Collagen prolyl 4-hydroxylases (C-P4H) are α2β2 tetramers, which catalyze the prolyl 4-hydroxylation of procollagen, allowing for the formation of the stable triple-helical collagen structure in the endoplasmic reticulum. The C-P4H α-subunit provides the N-terminal dimerization domain, the middle peptide-substrate-binding (PSB) domain, and the C-terminal catalytic (CAT) domain, whereas the β-subunit is identical to the enzyme protein disulfide isomerase (PDI). C-P4Hs are Fe(II) and 2-oxoglutarate-dependent dioxygenases, which use molecular oxygen to hydroxylate proline residues that are present at the Y position of the -X-Y-Gly- repeats of the procollagen chain. Studies have shown that the β/PDI subunit is required for providing the soluble and catalytically competent conformation of the α-subunit, but it is not understood how it is assembled with the α-subunit, how it is involved in intersubunit disulfide bridges, and what its role is in the procollagen hydroxylation reaction mechanism of the mature C-P4H α2β2 tetramer.

Here, we report on the characterization of two truncated human C-P4H-II variants in which the α-subunit is lacking either the N-terminal dimerization domain (C-P4H-II-Δ140) or the dimerization domain and the PSB domain (C-P4H-II-Δ281). The asymmetric unit consists of two C-P4H-II-Δ281 complexes, which are formed by the CAT domain of the α subunit, complexed with the complete β/PDI subunit. The N-terminal region of the α-subunit of the C-P4H-II-Δ281 complex, residues 284–328, which was previously proposed to be part of the linker region between the PSB and CAT domains, is actually an integral part of the CAT domain. This unique N-terminal extension of the CAT domain, not seen in any other P4H family member, forms two short α-helices (α12 and α13) followed by an extra β-strand (β1, including Cys311) of the major sheet of the DSBH-fold and another short α-helix (α14, including Ile324), before continuing into the secondary structure elements known from the other P4H structures. The structure of the C-P4H-II-Δ281 complex shows that in the CAT domain there is an intrasubunit disulfide bridge between two conserved cysteines, Cys294 (of the N-terminal extension of the CAT domain, in the α12-helix) and Cys504, located in β-strand βVII of the DSBH-fold. The assembly of the CAT-PDI heterodimer complex is stabilized by interactions of the unique N-terminal and C-terminal extensions of the CAT domain with the a’, b’, and a domains of PDI, whereas there are no interactions between the CAT domain and the b domain. The CAT-PDI protein–protein interfaces near Cys311 and Cys529 (of the CAT domain) include disulfide bridges with Cys397 and Cys53 (of PDI), respectively, which are the proximal cysteines of the CGHC motifs of the a’ and a domains. The third important interface between the CAT domain and the β/PDI subunit concerns the hydrophobic interactions of the Ile324 side chain of the CAT domain with the hydrophobic pocket of the PDI b’ domain.

>[2x]MHHHHHHMDYLPERDVYESLCRGEGVKLTPRRQKRLFCRYHHGNRAPQLLIAPFKEEDEWDSPHIVRYYDVMSDEEIERIKEIAKPKLARATVRDPKTGVLTVASYRVSKSSWLEEDDDPVVARVNRRMQHITGLTVKTAELLQVANYGVGGQYEPHFDFSRNDERDTFKHLGTGNRVATFLNYMSDVEAGGATVFPDLGAAIWPKKGTAVFWYNLLRSGEGDYRTRHAACPVLVGCKWVSNKWFHERGQEFLRPCGSTEVD;>MDAPEEEDHVLVLRKSNFAEALAAHKYLLVEFYAPWCGHCKALAPEYAKAAGKLKAEGSEIRLAKVDATEESDLAQQYGVRGYPTIKFFRNGDTASPKEYTAGREADDIVNWLKKRTGPAATTLPDGAAAESLVESSEVAVIGFFKDVESDSAKQFLQAAEAIDDIPFGITSNSDVFSKYQLDKDGVVLFKKFDEGRNNFEGEVTKENLLDFIKHNQLPLVIEFTEQTAPKIFGGEIKTHILLFLPKSVSDYDGKLSNFKTAAESFKGKILFIFIDSDHTDNQRILEFFGLKKEECPAVRLITLEEEMTKYKPESEELTAERITEFCHRFLEGKIKPHLMSQELPEDWDKQPVKVLVGKNFEDVAFDEKKNVFVEFYAPWCGHCKQLAPIWDKLGETYKDHENIVIAKMDSTANEVEAVKVHSFPTLKFFPASADRTVIDYNGERTLDGFKKFLESGGQDGAGDDDDLEDLEEAEEPDMEEDDDQKAVKDEL[2x]>MGHHHHHHHHHHGLVPRGSHMENVDLVIDLQFGSTGKGLIAGYLAEKNGYDTVINANMPNAGHTYINAEGRKWMHKVLPNGIVSPNLKRVMLGAGSVFSINRLMEEIEMSKDLLHDKVAILIHPMATVLDEEAHKKAEVGIATSIGSTGQGSMAAMVEKLQRDPTNNTIVARDVAQYDGRIAQYVCTVEEWDMALMASERILAEGAQGFSLSLNQEFYPYCTSRDCTPARFLADMGIPLPMLNKVIGTARCHPIRVGGTSGGHYPDQEELTWEQLGQVPEL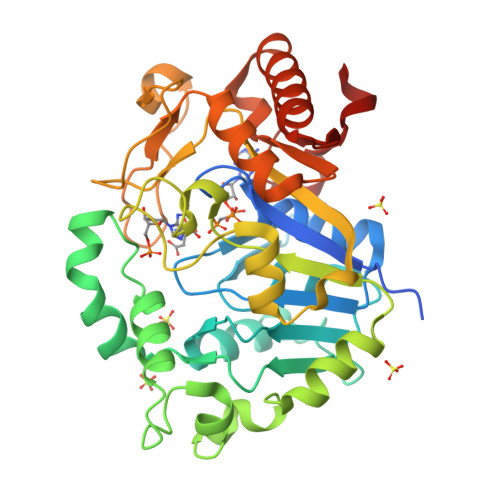TTVTKKVRRVFSFSFIQMQKAMWTCQPDEVFLNFCNYLSPMGWQDIVHQIEVAAQSRYCDAEVKYLGFGPTFNDVELREDVM[2x]1-beta-D-glucopyranosyl-4-naphthalen-2-yl-1H-1,2,3-triazole | C18 H19 N3 O5 | 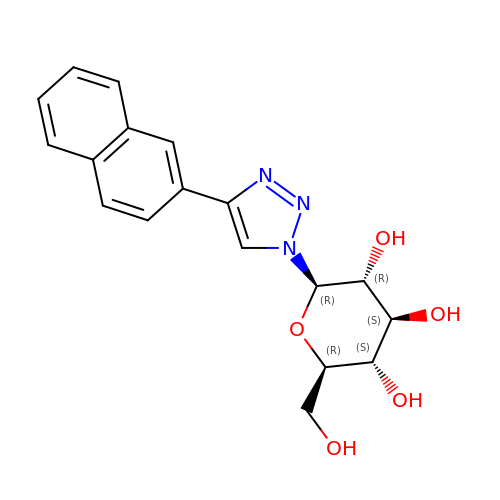BQMXQDYTYFMQSE-UYTYNIKBSA-N(2R)-3-oxo-2-(phosphonooxy)propanoic 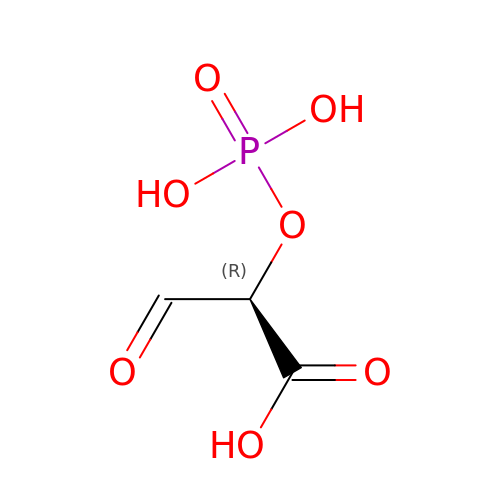acid | C3 H5 O7 P | KBLQTRXAGCIRPZ-UWTATZPHSA-N PII proteins are key sensors for the metabolic nitrogen status. Af-GlnK3 shares the canonical fold of PII proteins, consisting of a four-stranded, antiparallel beta sheet and two connecting alpha helices. It forms a tightly packed trimer with approximate dimensions of 30×54 Å. GlnK proteins, when activated, are sequestered to the cytoplasmic membrane where they bind directly to their corresponding Amt proteins, physically blocking ammonium uptake by inserting the T-loops deeply into the transporters' substrate channels.

2-OG bound to Af-GlnK3 with high affinity, but it did so exclusively in the presence of ATP and Mg2+. In the presence of 2-OG, a Mg2+ ion is clearly identified in the binding pocket by its near perfect octahedral coordination. Its ligands are three oxo groups from all three phosphates of ATP (thereby discerning ATP form ADP), and one α-carboxy oxygen atom and the α-keto-oxygen of 2-OG. The γ-amido oxygen atom of residue Gln 39 completes the six-fold coordination. In Af-GlnK3 the T-loops shift to attain a highly ordered β-hairpin conformation stabilized by six hydrogen bonds involving peptide amides, and are fully ordered in the crystal structure. Residue Arg 47 that is crucial for insertion into the substrate channels of the Amt protein upon complex formation, remains poised at the apex of the loop. However, 2-OG is fixed at the base of the loop in a wedge-like manner and pushes the T-loops outward with respect to their conformation in the ADP-bound state. In both structures, the Cα atoms of residue Arg 47 form an equilateral triangle, but while the sides of this triangle in a complex with the Amt protein have a length of 31 Å, they are extended to 46 Å in the form with bound 2-OG. They thus lose their structural flexibility and are pried apart too far to be able to insert into the substrate exit channels of Af-Amt3. Under conditions of sufficient energy and nitrogen, both ATP and 2-oxoglutarate levels will be high and the GlnK protein will reside in this blocked state.

>[3x]MKMVVAVIRPEKLECVKKALEERGFVGMTVTEVKGRGEQKGIRLQFRGREVEVDLLQKTKVEVVVSDDAVDEVVEAIVSSARTGKFGDGRIFVIPVEKSVKIRTGDEEVAAAHHHHHH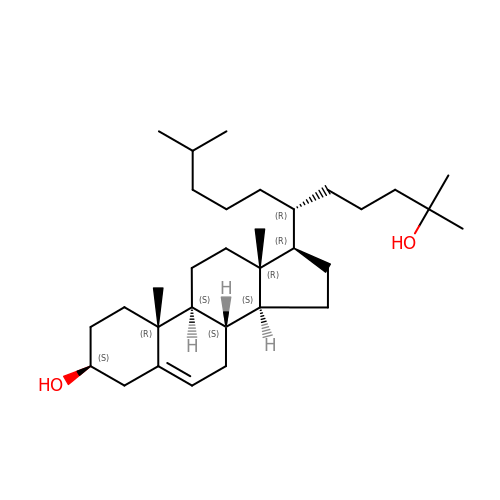(3~{S},8~{S},9~{S},10~{R},13~{R},14~{S},17~{R})-17-[(6~{R})-2,10-dimethyl-2-oxidanyl-undecan-6-yl]-10,13-dimethyl-2,3,4,7,8,9,11,12,14,15,16,17-dodecahydro-1~{H}-cyclopenta[a]phenanthren-3-ol | C32 H56 O2 | MDQUOZBEMDXUCO-PTHRTHQKSA-N>MISSFEVRKATIDDYFELRNLICDVTRCTETLSREQAEERFRYNTYHPYCLVDTENGRIVGYAGFYIIPHLGRKNDSRIEHVIISKEYRNRGLGRLLCKQIIEDAKNKFNCGRIDLTVESHIAKKLYSSLEFEKVNTEVMRNSFLDLTPKSD[2x]

GNA1 catalyzes the acetylation of glucosamine-6-phosphate (GlcN6P) to generate N-acetylglucosamine-6-phosphate (GlcNAc6P), which is needed for the biosynthesis of UDP-GlcNAc, a required precursor for both GPI-anchors and N-glycans. Apicomplexan parasites have a hexosamine pathway comparable to other eukaryotic organisms, with the exception of the glucosamine-phosphate N-acetyltransferase (GNA1) enzymatic step that has an independent evolutionary origin and significant differences from nonapicomplexan GNA1s. To further characterize the enzyme and, given our inability to express and purify sufficient amounts of active PfGNA1 (10), we used CpGNA1 as a surrogate, considering that it belongs to the same Apicomplexa-specific GNA1 family and can be purified fairly well with a high yield. CpGNA1 is found as a dimer, as is the case for other reported GNA1 crystal structures. CpGNA1 adopts the typical GCN5-related N-acetyltransferase (GNAT) fold previously described in GNA1 enzymes, though with some variations (see below).

The dimeric structure of CpGNA1 in complex with acetyl-CoA and glucose-6-phosphate (Glc6P) from data at 1.95 Å in space group P212121 was solved by molecular replacement with Phaser using the monomeric structure, and further assessing ligand binding by representing unbiased sim-omit maps. Note that Glc6P was used previously as a pseudosubstrate to get insights into GNA1-GlcN6P recognition and catalysis. The CpGNA1 structure consists of a central twisted four-stranded antiparallel β-sheet surrounded by four α helices. Remarkably, the highly conserved tyrosine of the active site, also present in CpGNA1 (Tyr127), establishes a hydrogen bond between its hydroxyl group and the thioester sulfur, leading to an increase in the electrophilic character of the carbonyl group of the acetyl-CoA molecule during catalysis. Note the proximity of the Glc6P OH2 that mimics the amine group of GlcN6P to the carbonyl group of acetyl-CoA (distance of 3.45 Å), which clearly supports that the same mechanism might take place for CpGNA1. There are 19 residues of CpGNA1 engaged in the recognition of acetyl-CoA and Glc6P. The adenine moiety and the dimethyl group of acetyl-CoA establish CH-π and CH-CH interactions with Ile122 and Ala123/Leu126, respectively. The phosphorylated ribose, pyrophosphate, pantothenic acid, the β-mercaptoethylamine, and the acetyl moieties are tethered via hydrogen bonds to the Arg95 side chain and Lys125 backbone, Asn90/Arg91/Gly92/Gly94/Arg95 backbones, Ile84 backbone, Val82 backbone, and His81/Val82 backbones, respectively. The Glc6P is tethered via hydrogen bonds to the His81/Thr117/Arg27 backbones and Arg73B/His81/Arg113B/Thr117 side chains.> MNSTPKGTIYLTFDDGPVNASVEVIKVLNQGGVKATFYFNAWHLDGIGDENEDRALEALKLALDSGHIVGNHSY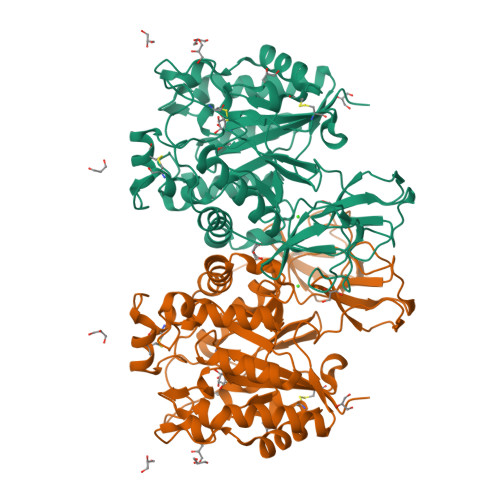DHMIHNCVEEFGPTSGADCNATGNHQIHSYQDPVRDAASFEQNLITLEKYLPTIRSYPNYKGYELARLPYTNGWRVTKHFQADGLCATSDNLKPWEPGYVCDPANPSNSVKASIQVQNILANQGYQTHGWDVDWAPENWGIPMPANSLTEAVPFLAYVDKALNSCSPTTIEPINSKTQEFPCGTPLHADKVIVLTHDFLFEDGKRGMGATQNLPKLAEFIRIAKEAGYVFDTMDNYTPRWSVGKTYQAGEYVLYQGVVYKAVISHTAQQDWAPSSTSSLWTNADPATNWTLNVSYEQGDIVNYKGKRYLVSVPHVSQQDWTPDTQNTLFTALELRRQWSHPQFEK>[2x]MQINIQGHHIDLTDSMQDYVHSKFDKLERFFDHINHVQVILRVEKLRQIAEATL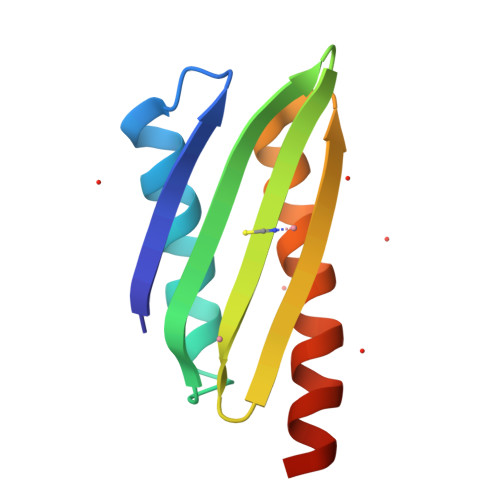HVNQAEIHAHADDENMYAAIDSLVDKLVRQLNKHKEKLSSH>MASGTDTGRFSRNLKD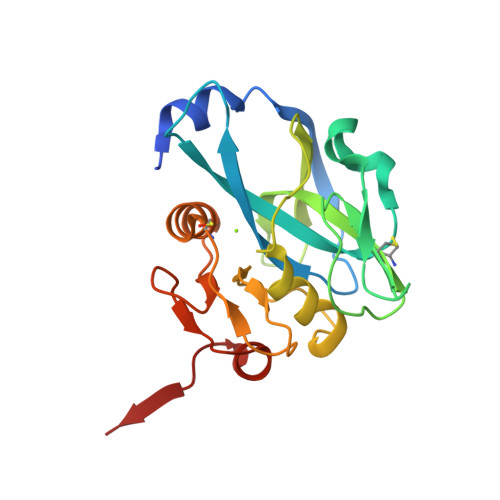RLESNNYEEMELPPPTKGVIIPVVHTVESAPGEAFGSLLVIIPGAYPELLDPNQQVLSHFKNDTGCVWGIGEDIPFEGDDICYTALPLKEIKKNGNIVVEKVFAGPAMGPSCQLGLSLLVNDIDKGVPRMVFTGEIANDEETIVPICGVDIAAIAAHEHGLPLVGCQPGVDEVVANTSLASHLIQSGALPVQKA[2x]>DVKIEKLKDNLYVYTTYNTFNGTKYAANAVYLVTDKGVVVIDCPWGEDKFKSFTDEIYKKHGKKVIMNIATHSHDDRAGGLEYFGKIGAKTYSTKMTDSILAKENKPRAQYTFDNNKSFKVGKSEFQVYYPGKGHTADNVVVWFPKEKVLVGGCIIKSADSKDLGYIGEAYVNDWTQSVHNIQQKFSGAQYVVAGHDDWKDQRSIQHTLDLINEYQQKQKASN[4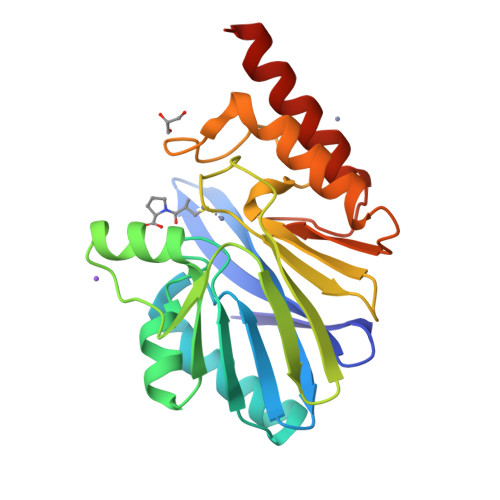x]>MNVLVIEDDKVFRGLLEE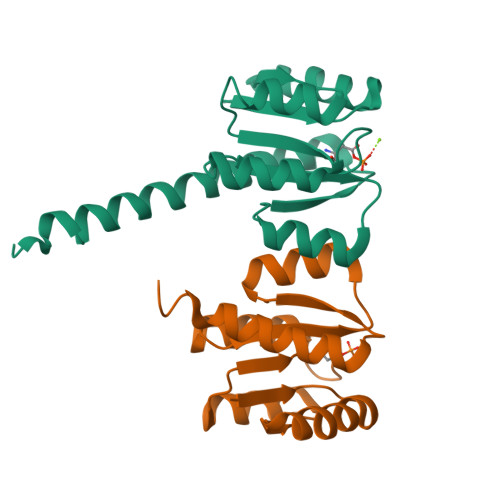YLSMKGIKVESAERGKEAYKLLSEKHFNVVLLDLLLPDVNGLEILKWIKERSPETEVIVITGHGTIKTAVEAMKMGAYDFLTKPCMLEEIELTINKAIEHRKLRKENELLRREKDLKEKLAAALEHHHHHHH[2x]>[2x]TRDQNGTWEMESNENFEGYMKALDIDFATRKIAVRLTQTKVIDQDGDNFK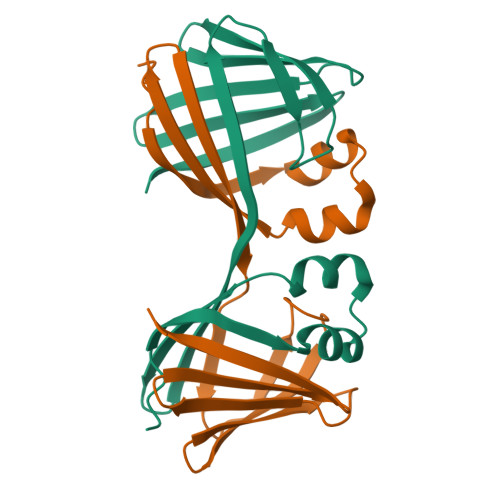TKTTSTFRNWDVDFTVGVEFDEYTKSLDNRHVKALVTWEGDVLVCVQKGEKENRGWKQWIEGDKLYLELTCGDQVCRQVFKKK>[10x]MPLVGNKAPDFEAEAVFDQEFIKVKLSDYIGKKYVILFFYPLDFTFVSPTEITAFSDRHSEF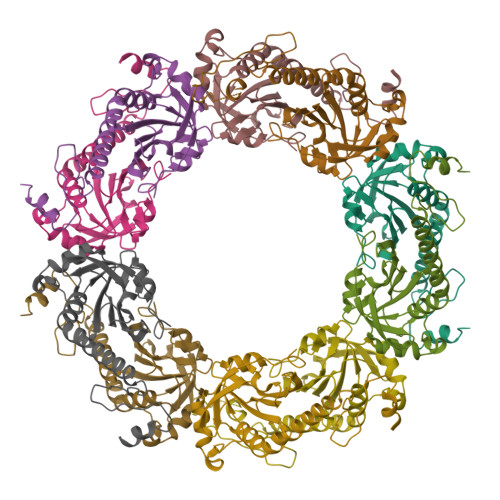EKLNTEVLGVSVDSVFSHLAWVQTDRKSGGLGDLNYPLISDVTKSISKSFGVLIHDQGIALRGLFIIDKEGVIQHSTINNLGIGRSVDETMRTLQALQYIQENPDEVCPAGWKPGEKSMKPDPKLSKEYFSAILEHHHHHH> KPQVTILATGGTIAGSGAVTVDKLLAAVPAINDLATIKGEQISSIGSQEMTGKVWLKLAKRVNELLAQKETEAVIITHGTDTMEETAFFLNLTVKSQKPVVLVGAMRPGSSMSADGPMNLYNAVNVAINKASTNKGVVIVMNDEIHAAREATKLNTTAVNAFASPNTGKIGTVYYG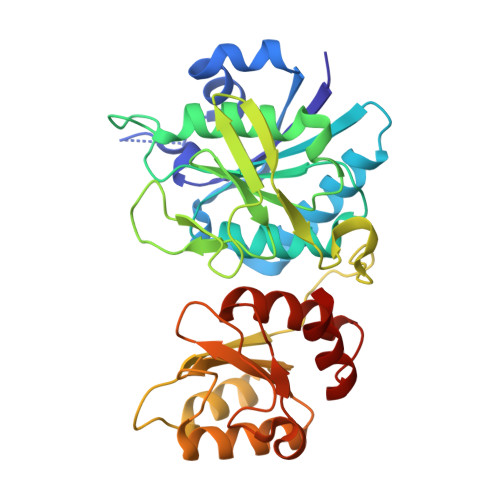KVEYFTQSVRPHTLASEFDISKIEELPRVDILYAHPDDTDVLVNAALQAGAKGIIHAGMGNGNPFPLTQNALEKAAKSGVVVARSSRVGSGSTTQEAEVDDKKLGFVATESLNPQKARVLLMLALTKTSDREAIQKIFSTY>[2x]MAPQMEKVSEELILPSSPTPQSLKCYKISHLDQLLLTCHIPFILFYPNPLDSNLDPAQTSQHLKQSLSKVLTHFYPLAGRINVNSSVDCNDSGVPFVEARVQAQLSQAIQNVV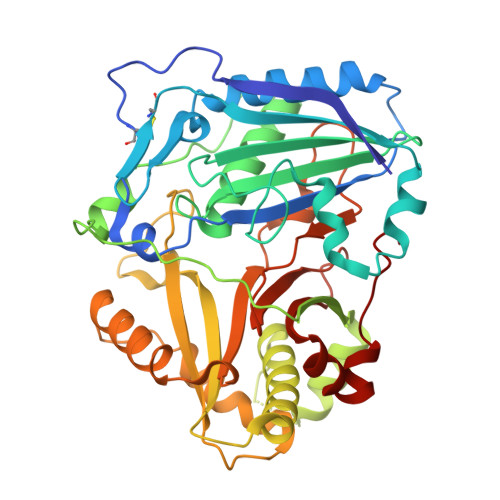ELEKLDQYLPSAAYPGGKIEVNEDVPLAVKISFFECGGTAIGVNLSHKIADVLSLATFLNAWTATCRGETEIVLPNFDLAARHFPPVDNTPSPELVPDENVVMKRFVFDKEKIGALRAQASSASEEKNFSRVQLVVAYIWKHVIDVTRAKYGAKNKFVVVQAVNLRSRMNPPLPHYAMGNIATLLFAAVDAEWDKDFPDLIGPLRTSLEKTEDDHNHELLKGMTCLYELEPQELLSFTSWCRLGFYDLDFGWGKPLSACTTTFPKRNAALLMDTRSGDGVEAWLPMAEDEMAMLPVELLSLVDSDFSK>MRYEEAGVHIEAKAEALRRAREAIAATYTPEVLRGMGAFGGLYAASRLKALEEPVLVATTDGVGTKTLLALEAGDVSGLGFDLVNHSVNDLLAQGAEPLFFLDYLAASHLDEGVLAALLASLAEACRAHGIPLLGGETAEMPGVYREG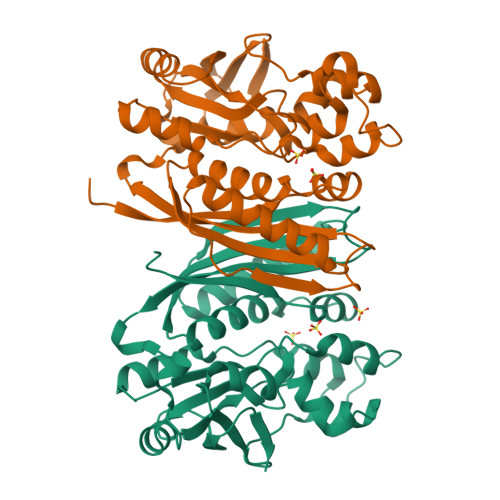AWDIAGTLVGVVERSRILGPERVREGDALLALPSSGPHTNGYSLIRKVVAGQDLSAPVPELGESLKEALLRPHRAYLKEFRLLWEAGVELHAAAHITGGGLPENLPRALPPGLGAEVRRGSWPIPPVFPYLQRLGGIPEEEMYRVFNMGLGMVLVLPQEAAEEALKLVEGFLVGRVVPGEGVRLV[8x]(~{E})-2-(1,3-benzoxazol-2-yl)-3-[4-[2-hydroxyethyl(methyl)amino]phenyl]prop-2-enenitrile 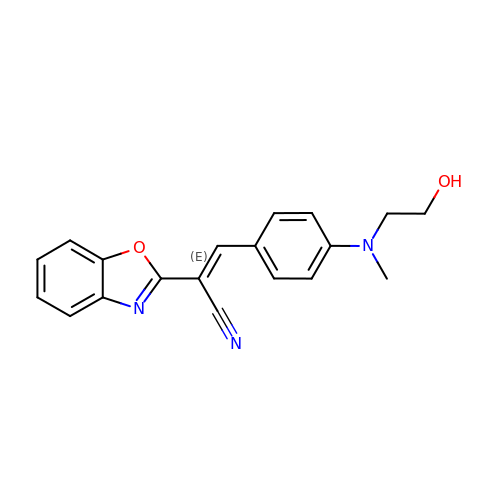| C19 H17 N3 O2 | PARAUTMXYRINAC-NTCAYCPXSA-N> ANFMIYPISKDLKNGNSELVRVYSKSKEIQYIKIYTKKI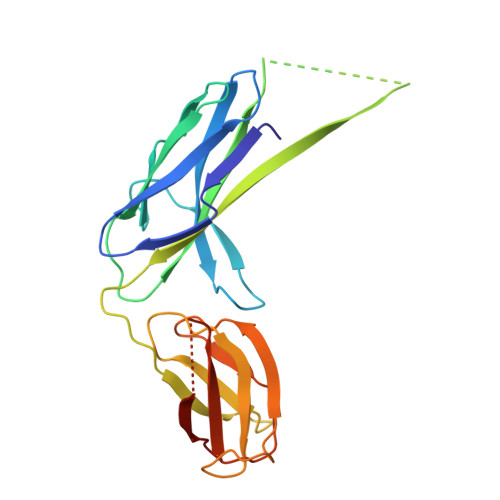INPGTTEEYEVDIPNWDGGLVVTPQKVILPAGASKSIRLTQFKIPKKEEVYRVYFEAVKPDSKENVIDNKKLTIEISINIIYAALIRSLPSEQNISLNISRNAKKNIIIYNNGNVRAGVKDIYFCKSSNIDDNCVKKAYNKNIYPEKSFDTLVNNNFSYVFIKLNHEGIEKEQGLIQLKVPA R2R3-MYB proteins only exist in terrestrial plants, but they form the largest subfamily of MYB transcription factors. R2R3-MYB proteins play important roles in metabolism, cell fate determination, growth and development, and responses to biotic and abiotic stress. In Arabidopsis roots, WER is specifically expressed in non-hair cells (N-cells) and activates GLABRA2 (GL2), a central regulatory gene for epidermal cell fate determination. Previous in vitro and in vivo studies showed that WER specifically recognizes the cis-element WER Binding Site (WBS) located within the GL2 promoter and inhibits root hair formation in N-cells.

Though crystals were only obtained in the presence of WER 12–130 (named WER-R2R3) and dsDNA, they diffracted well (up to 2.15 Å). WER-R2R3 is composed of six α-helices, H1 (V23–H36), H2 (W41–K47), H3 (G54–L65), H4 (E76–L89), H5 (W93–R99) and H6 (D105–L116). Helices H1–H3 and H4–H6 belong to the R2 and R3 repeats, respectively. The WER–DNA complex structure showed that the third helices (H3 and H6) of R2 and R3 are inserted into the major groove of the DNA, producing a sequence-specific interaction with the 5′-AACCGC-3′ motif. A10:T13* (the first base pair of the 5′-AACCGC-3′ motif) forms two H-bonds with N110 of R3; one (2.9 Å) is between the N7 atom of A10 and the ND2 atom of N110 and the other (3.0 Å) is between the N6 atom of A10 and the OD1 atom of N110. A11:T12* (the second base pair of the 5′-AACCGC-3′ motif) is also recognized by one Asn residue (N106), through two similar H-bonds between the nucleobase of A11 and the side chain of N106. The third base pair of the 5′-AACCGC-3′ motif, C12:G11*, is recognized by K109 of R3. The NZ atom of K109 forms H-bond interactions with both the O6 and the N7 atoms of G11*; the average distance is around 2.9 Å. G14:C9* and C15:G8* (the fifth and sixth base pairs of the 5′-AACCGC-3′ motif) are both recognized by K55 of R2. Owing to the presence of R52, R58, and R60, the outer surface of WER-R2R3 is highly positive, and the side chains of these positively charged residues form extensive H-bond interactions with DNA phosphate backbones.

> GNNEYKKGLWTVEEDKILMDYVKAHGKGHWNRIAKKTGLKRCGKSCRLRWMNYLSPNVKRGNFTEQEEDLIIRLHKLLGNRWSLIAKRVPGRTDNQVKNYWNTHLSKKLGIKDQKTKQS Transcription termination is an essential step in transcription by RNA polymerase (RNAP) and crucial for gene regulation. For many bacterial genes, transcription termination is mediated by the adenosine triphosphate–dependent RNA translocase/helicase Rho, which causes RNA/DNA dissociation from the RNAP elongation complex (EC). Rho is an adenosine triphosphate (ATP)–dependent RNA translocase/helicase with 5′ → 3′ directionality. Rho forms a ring-shaped homo-hexameric complex, mediated by the CTD.

Cryo-EM maps of Rho, apo RNAP, EC, and type 1 and type 2 complexes are shown. It consists of the N-terminal domain (NTD) and the C-terminal domain (CTD), which have the primary RNA binding site (PBS) and the secondary RNA binding site (SBS), respectively. The Rho hexamer can adopt both open- and closed-ring conformations. When Rho binds RNA and ATP, it assumes the closed-ring conformation to thread the RNA into its central channel composed of the SBS. The purified EC was mixed with Rho in the presence of ADP·BeF3 and cross-linked with BS3 to stabilize the complex before the preparation of cryo-grids.

>[6x]GPMRRKETLQETPLTYQELASKILPELHLLAQEAGIEGYKRMKKDQLIMALLERQTQGEGLRLVKGYLEISQDGYGFLTENLHNLESRVAIVSAGLIKQYALRAGDYVVGQARPPRENERYATLLKVEAVNNLDPEAAKNRPRFDELTPQFPDRQIRLETTPDELSTRVIDLLAPIGRGQRGLIVAPPKAGKTTLLKKIANAVLKNEPDIKVIVLLIDERPEEVTDFRESVQGAEVIASTFDEPPQNHIRVAEFVHERAKRIVEEGGHVMILLDSITRLARANNLVTPPTGRTLSGGLDSAALYFPKRFLGAARNIRGGGSLTILATALVETGSRMDDVIFEEFKGTGNMELHLSRRLEERRIFPAIDILKSGTRREELLLGEEVTHKMWLLRKVLADMDPAEAMEMLLARLARTKNNKEFLASLAAR> EGYGKHITSMHVRNIFNQGNQVIRNIVKQQRYELLDFTGTEAGTTNLPKIIPYQCIWWRGLQNAANVNQTINNMIALNTISYGVRFLKAKLCIEVYAVTRKRLIQTGATSYYTDDFEQGQNLFIGWADRKAESIPITTPADLDETKLTVANTTLFDANNDNITKEEVPTREKWCHTWDLDVLNHNYLWEPNNLDSQWTLIPGAQAVQPTATPIGPTYQEIVIATKAIGANESALVTTIQDRRSYPRLMLSQPQIKDETDTMKFKYQIRISTELEMEHHIKPDIANPWLTRQTLPLPALSGDGTTRYVPCVPYETHVSQ

We report the discovery of a parvovirus with a bipartite genome, Acheta domesticus segmented densovirus (AdSDV), isolated from house crickets (Acheta domesticus), in which it is pathogenic. Our structural and molecular examinations revealed that the AdSDV packages one genome segment per particle. The AdSDV capsid displayed an overall “smooth” capsid surface with the only protruding area surrounding the fivefold symmetry axis. The AdSDV VP subunit displayed the canonical eight-stranded jelly roll fold, complemented by an N-terminal βA, located on an elongated N-terminal region.

The subsequent sucrose gradient had two distinct particle bands; in the 20% fraction (empty capsids, EC), and in the 25% fraction (genome containing “full” capsids, FC). Cryoelectron microscopy (cryo-EM) micrographs revealed that the consistently high genome count of the FC population (in the range of >1015 genome particles of each segment) is indeed due to the presence of almost exclusively full, genome-packaging particles. This number was multiple logs lower in case of the EC capsids, which displayed an overwhelmingly large proportion of empty capsids. The interior of the FC was filled with density attributed to the ssDNA genome. The slight amount of genome-like density of EC capsid interior confirmed the genome quantification and EM results, namely that this population is heterogenous and is composed of EC1, EC2 and FC capsids (detailed by Fig. S7). The EC, EC1, EC2 and the ORF1-VLPs monomer lacked two N-terminally ordered residues as well as the unusually elongated C-terminal tail of the FC population, making Gln366 the last ordered residue. The AdSDV fivefold channel displayed two distinct conformation states i.e., either an “empty” for the EC fractions and the vpORF1-VLPs, or “filled” as observed in the FC population. In contrast, both EC populations displayed DE loops pointing inwards, narrowing the pore from 16.0 Å (FC) to 10.1 Å, with Tyr159 and Ile152 retracted underneath the DE loop peak.>GSHMASQVGVIKPWLLLGSQDAAHDLDTLKKNKV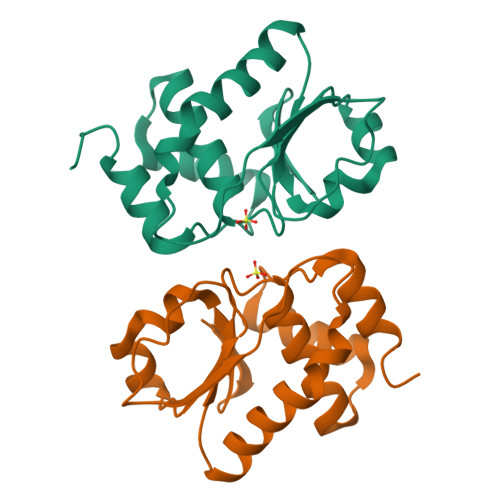THILNVAYGVENAFLSDFTYKSISILDLPETNILSYFPECFEFIEEAKRKDGVVLVHSNAGVSAAAAIVIGFLMNSEQTSFTSAFSLVKNARPSICPNSGFMEQLRTYQEGKE[2x]~{N}-(1-propyl-1,2,3,4-tetrazol-5-yl)furan-2-carboxamide | C9 H11 N5 O2 | 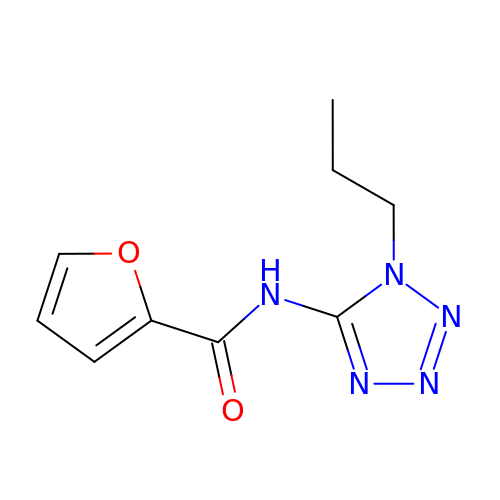XGSKVFLLSUZGMA-UHFFFAOYSA-N> EMAESVTNPQRPPVIWIGAQECTGCTESLLRATHPTVENLVLETISLEYHEVLSAAFGHQVEENKHNALEKYKGQYVLVVDGSIPLKDNGIYCMVAGEPIVDHIRKAAEGAAAIIAIGSCSAWGGVAAAGVNPTGAVSLQEVLPGKTVINIPGCPPNPHNFLATVAHIITYGKPPKLDDK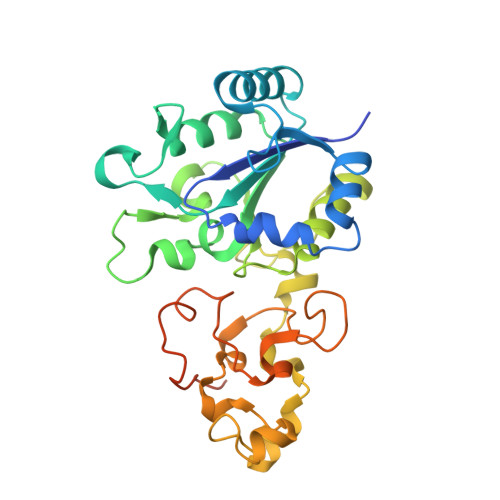NRPTFAYGRLIHEHCERRPHFDAGRFAKEFGDEGHREGWCLYHLGCKGPETYGNCSTLQFCDVGGVWPVAIGHPCYGCNEEGIGFHKGIHQLANVENQTPRSQKPDVNAKEGGRSHHHHHH>[16x]MYEWKLNDIVDNGICAKCGTCTVVCPNGILTFEDRPKLTEECLRKGNGMCFEVCPRVSSGKYQIKIREKFKEEYYYGKGDVEGQDGGVVTTFLKYLLKNKKIDGAIVVGDECWKPVSLIVQNEEDLMNTTKSKYTVSTLEALKTAGEMGLEKVAVVGLPCQINGLRKLQYFQYLAKHDGELGKNGKPVKLPKIEYLIGLLCTEKFEYDELKETLAKYNINMDDVEKFDIKKGKLLVYVNGEEHKIPLKEIELSAGCKMCRDFDAEMADVSVGCVGSPDGYSTVIIRTEKGEEIKNAIELKEGVNLEAIEKLRDLKLNRFKKEVERRKAEDEKVSFYWTADYGGVGKRADGTYFIRIRAKPAGWYSIDEAREILEIAEKYDGKIKMTNRGAFEIHGISGFDVEAMVLELMEKGFITGSEGPLVRATLACPGEGNCGSGLINTTELCKILEDNFKEHPAPYKFKIAISGCPNKCVRPQIHDIGIAGVKFPVVNEENCNGCGRCAEVCKIEAIDIRGETSYTNYNVCIGCGKCIKACPNEGRDVKEEGFMVYVGGKTGREVIEGVSMKLMSVEEILNLIDKVLIVYHKYAKKPQRERLAAVMARIGKGKFLEEVKELMEQN

Here, we present snapshots of this coupled system, named coenzyme F420-dependent sulfite reductase (Group I Fsr), obtained from two marine methanogens. Fsr organizes as a homotetramer, harboring an intertwined six-[4Fe–4S] cluster relay characterized by spectroscopy. The wire, spanning 5.4 nm, electronically connects the flavin to the siroheme center. Despite a structural architecture similar to dissimilatory sulfite reductases, Fsr shows a siroheme coordination and a reaction mechanism identical to assimilatory sulfite reductases.

MtFsr was solved by molecular replacement, using MjFsr as a template. Notably, the asymmetric unit of MtFsr contains four tetramers (including 96 [4Fe–4S] clusters), providing insights on its natural flexibility. Fsr is organized as follows: the N-terminal ferredoxin domain (MtFsr residues 1–57 containing two [4Fe‒4S] clusters) is linked to the F420H2-oxidase domain (MtFsr residues 58–336, harboring the flavin and one [4Fe‒4S] cluster), which is connected to the C-terminal sulfite reductase domain (MtFsr residues 339–484, 546–618) that binds the siroheme‒[4Fe‒4S] and has an inserted ferredoxin domain (MtFsr residues 485–545, containing two [4Fe‒4S] clusters). The extended loop 171–189 in Fsr serves as a platform to specifically bind both ferredoxin domains, and the Glu 180 coordinates the [4Fe‒4S] cluster 3 (monodentate, 2.22 Å). In MtFsr, the axial ligand is a single atomic species at all sites of the asymmetric unit, which is in proximity but not covalently bound to the iron (2.9 Å). The anion HS− was modeled in the electron density based on the pH 5.5 in the crystallization solution. This species could be the result of cocrystallizing Fsr with reduced F420, which might have forced the complete reduction of bound SO32−. In MtFsr, the modeled HS− is bound by Arg 423, Lys 460 and Lys 462, and one water molecule is stabilized by Arg 355. MtFsr did not accept thiosulfate as an electron acceptor, which is in agreement with the findings for MjFsr5. In addition, we have shown that MtFsr reduces selenite (SeO32−) in vitro with a relative activity of 20.7 ± 7.5% compared to SO32−.>[2x]GSPIGIHMSGQSLTDRITAAQHSVTGSAVSKTVCKATTHEIMGPKKKHLDYLIQCTNEMNVNIPQLADSLFERTTNSSWVVVFKSLITTHHLMVYGNERFIQYLASRNTLFNLSNFLDKSGLQGYDMSTFIRRYSRYLNEKAVSYRQVAFDFTKVKRGADGVMRTMNTEKLLKTVPIIQNQMDALLDFNVNSNELTNGVINAAFMLLFKDAIRLFAAYNEGIINLLEKYFDMKKNQCKEGLDIYKKFLTRMTRISEFLKVAEQVGIDRGDIPDLSQAPSSLLDALEQHLASLEGKK

Here, we show that the R-SNAREs VAMP8, VAMP3, and VAMP2, which cycle between the plasma membrane and endosomes, bind directly to the ubiquitously expressed, PtdIns4,5P2-binding, endocytic clathrin adaptor CALM/PICALM. X-ray crystallography shows that the N-terminal halves of their SNARE motifs bind the CALMANTH domain as helices in a manner that mimics SNARE complex formation. In this study, we provide structural, biochemical and in vivo data to show that the internalization of VAMP8, and consequently that of the highly related small R-SNAREs, VAMP3 and VAMP2, is mediated by specific, direct interactions between the N-terminal halves of their SNARE motifs and the ANTH (AP180 N-terminal Homology) domain of the endocytic clathrin adaptor CALM. Thus, CALM:R-SNARE interactions ensure that R-SNAREs, required for the fusion of endocytic clathrin-coated vesicles with endosomes and also for subsequent postendosomal trafficking, are sorted into endocytic vesicles.

Attempts were made to crystallize a complex of CALMANTH with a peptide corresponding to residues 10–41 of VAMP8, both with the two components free in solution and with residues 10–41 of VAMP8 appended on the C terminus of CALMANTH. While these cocrystallizations did not yield the structure of a complex, they did yield a 1.8Å resolution structure (final R/Rfree 0.182/0.216) of the unliganded ANTH domain with two molecules in the asymmetric unit. In both molecules the positions of the first ten helices are identical. The CALMANTH structures presented here in conjunction with the previously published structure (Ford et al., 2001) suggested that residues 265–289 of CALM are not integral to the ANTH domain but are flexible and associate only weakly with the domain's core residues (19–264). Inspection of the CALMANTH surface showed that the elongated patch on which the ordered short helix 11 and preceding ten residues of CALM sat was hydrophobic in nature and of the correct dimensions to bind an α helix and was thus a good candidate for the interaction site for the hydrophobic SNARE motif of a VAMP. In order for a small R-SNARE VAMP to bind to CALMANTH, helix 11 of the ANTH domain must be displaced. This dissociation will be facilitated by the fact that helix11 is only poorly associated with the rest of the ANTH domain (helices 1–10) and may be further modulated by the C-terminal tail of CALM that follows helix11 binding to the clathrin terminal domains that are displayed on the underside of the polymeric clathrin lattice (Morgan et al., 2000).> SPGQGTQSENSCTHFPGNLPNMLRDLRDAFSRVKTFFQMKDQLDNLLLKESLLEDFKGY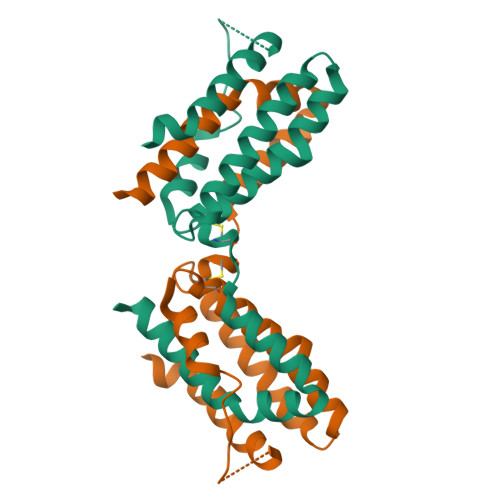LGCQALSEMIQFYLEEVMPQAENQDPDIKAHVNSLGENLKTLRLRLRRCHRFLPCENKSKAVEQVKNAFNKLQEKGIYKAMSEFDIFINYIEAYMTMKIRN>AEQKTLHIYNWTDYIAPDTVANFEKETGIKVVYDVFDSNEVLEGKLMAGSTGFDLVVPSAYLLERQLTAGVFQPLDKSKLPEWKNLDPELLKLVAKHDPDNKFAMPYMWATTGIGYNVDKVKAVLGENAPVDSWDLILKPENLEKLKSCGVSFLDDPEEVFATVLNYLGKDPNSTKADDYTGPATDLLLKLRPNIRYFHSSQYINDLANGDICVAIGWAGDVWQASNRAKEAKNGVNVSFSIPKEGAMAWFDVFAMPADAKNKDEAYQFLNYLLRPDVVAHISDHVFYANANKAATPLVSAEVRENPGIYPPADVRAKLFTQKVQDPKIDRVRTRAWTKVKSGKLEHHHHHH[2x]

To gain insight into the evolution and designability of ligand binding and specificity, we analyzed the homologous PBPs, PotF and PotD, which are Escherichia coli putrescine (PUT)-binding protein and spermidine (SPD)-binding protein, respectively. They constitute the first elements of two separate multicomponent uptake systems (PotFGHI and PotABCD) to transport the cationic polyamines PUT and SPD across the cellular membrane. Still, the protein-binding modes differ: PotF shows affinity for PUT and SPD, whereas PotD exclusively binds SPD. Prior to this work, we grafted the seven differences in amino acids from PotD binding pocket onto PotF; this resulted in PotF_SPD, which will be referred to as PotF/D throughout this work to keep naming for mutants more concise.

We introduced the S247D exchange into PotF/D and into our high-affinity constructs E39D–Y87S–F88Y and E39D–F88A/L. The combination of S247D with the other constructs led to an affinity improvement with which the nanomolar range was reached for the first time, while keeping the order of affinities in the different mutants the same compared with the prior analysis. All structures but PotF/D–S247D adopt a fully closed wildtype conformation. In the F88L/A variants, Y87 is finally able to rotate toward the binding pocket and allows distal salt bridge formation. The orientation of the residues in both mutants is identical, confirming the F88L containing variant as a structural example for the noncrystallizable F88A construct in the first part of this study. Chain B as well as the A–B chain comparison behaves in a comparable manner. This deviation puts extra strain on the structure of F88L and especially the distal salt bridge since R91 is in the affected region. In general, the noise in the Fo–Fc map of this structure seems to indicate many flexible side chains. The “flexible” F88L structure is also the first in which we ever observed SPD taking alternate conformations in the binding pocket of which one does not mimic PUT-like positioning.> SMQKLINSVQNYAWGSKTALTELYGIANPQQQPMAELWMGAHPKSSSRITTANGETVSLRDAIEKNKTAMLGEAVANRFGELPFLFKVLCAAQPLSIQVHPNKRNSEIGFAKENAAGIPMDAAERNYKDPNHAPELVFALTPFLAMNAFREFSDIVSLLQPVAGAHSAIAHFLQVPNAERLSQLFASLLNMQGEEKSRALAVLKAALNSQQGEPWQTIRVISEYYPDDSGLFSPLLLNVVKLNPGEAMFLFAETPHAYLQGVALEVMANSDNVLRAGLTPKYI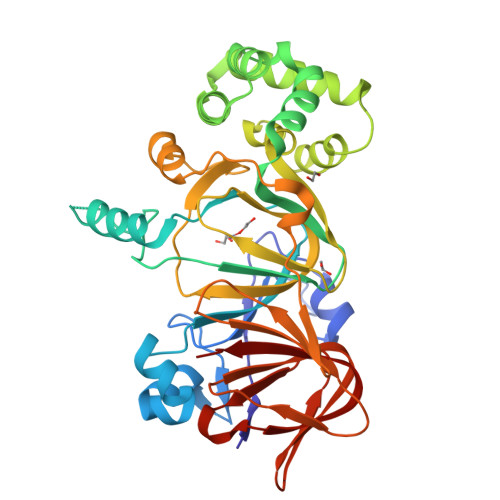DIPELVANVKFEPKPAGELLTAPVKSGAELDFPIPVDDFAFSLHDLALQETSIGQHSAAILFCVEGEAVLRKDEQRLVLKPGESAFIGADESPVNASGTGRLARVYNKL>SAHGLTDDMTMHFRMEGCVDGHKFVIEGNGNGNPFKGKQFINLCVIEGGPLPFSEDILSAAFDYGNRLFTEYPEGIVDYFKNSCPAGYTWHRSFRFEDGAVCICSADITVNVRENCIYHESTFYGVNFPADGPVMKKMTTNWEPSCEKIIPINSQKILKGDVSMYLLLKDGGRYRCQFDTIYKAKTEPKEMPDWHFIQHKLNREDRSDAKNQKWQ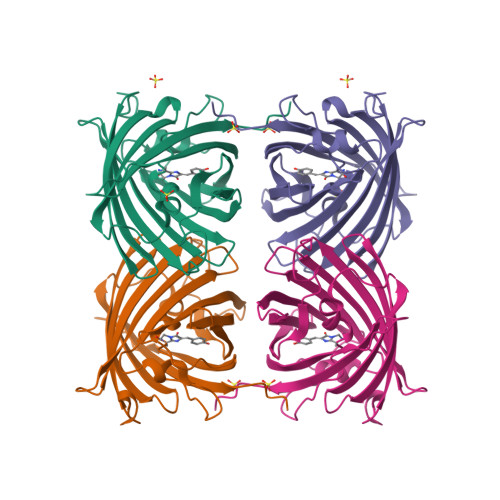LIEHAIASRSALP[4x]>[2x]MKKVYFNHDGGVDDLVSLFLLLQMDNVELTGVSVIPADCYLEPAMSASRKIIDRFGKNTIEVAASNSRGKNPFPKDWRMHAFYVDALPILNESGKVVTHVAAKPAHHHLIETLLQTEEKTTLLFTGPLTDLARALYEAPIIENKIKRLVWMGGTFRTAGNVHEPEHDGTAEWNSFWDPEAVARVWEANIEIDLITLESTNQVPL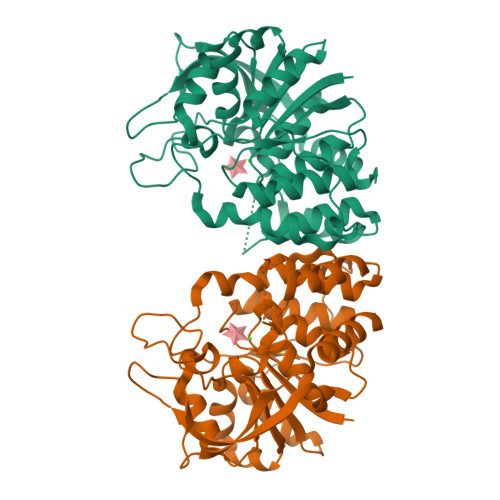TIDIREQWAKERKYIGIDFLGQCYAIVPPLVHFAKNSTYYLWDVLTAAFVGKADLAKVQTINSIVHTYGPSQGRTVETDDGRPVHVVYDVNHDRFFDYITRLAKKVST> MS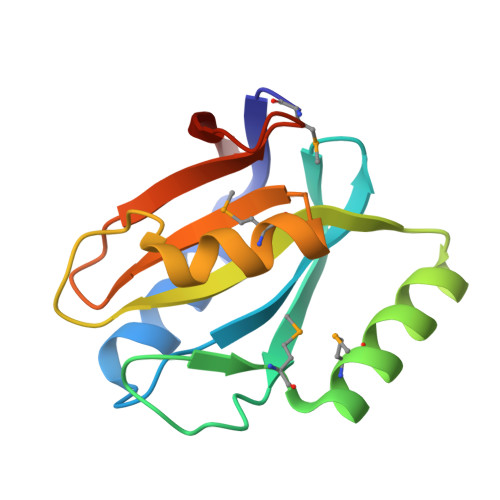TLIIPQHYLRAILKVVSSSSVEVCGFLFGKENRVLKVRFIRNRLNSPVEFEMDPEEMLKALEEAEQENLEVVGIFHSHIACPPIPSGKDLEGMKRWPVIWLIVNEKGEYKAWILSEKNKISEVKIVVE> TSSANEDMPVEKILEAELAVEPKTETYVEANMGLNPSSPNDPVTNICQAADKQLFTLVEWAKRIPHFSELPLDDQVILLRAGWNELLIASFSHRSIAVKDGILLATGLHVHRNSAHSAGVGA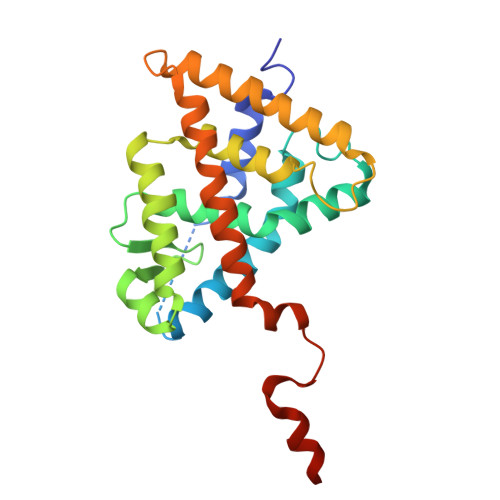IFDRVLTELVSKMRDMQMDKTELGCLRAIVLFNPDSKGLSNPAEVEALREKVYASLEAYCKHKYPEQPGRFAKLLLRLPALRSIGLKCLEHLFFFKLIGDTPIDTFLMEMLEAPHQAT> MMKIVVNNQSTLAAELMIVAQENLQKLVEQTKCPNSKALLDRRIFKAKSGEVLPLLHGDKIVILLGLGLRQDFIASEYDKIIAKAAEQLKKLAIKEISVDIDYAFENDNVKQFTLDTVRALISETYVFDQLKTEKENYSLEQIELVYSGDQDIEDSAKIGSAIACG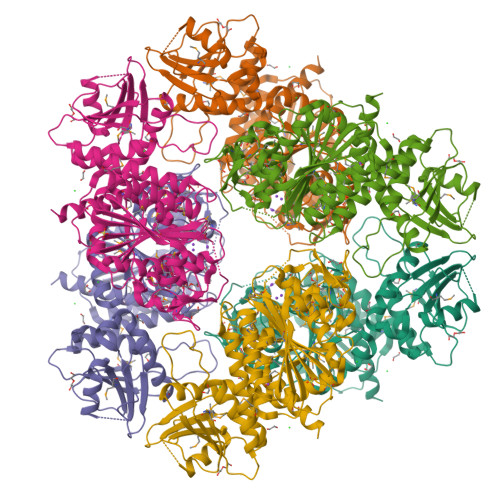QNYAKDLQNLPANICTTDYMLNEARELTSKYATFSLDYLDQDAMAELGMGCALAVGRGSYMSNYTVCMEYKGGNEGDAPIVLVGKGLVFDNGGICIKQAAGMDSMKMDMGGVAAVMGTMKAIAMLNLPVNVVGVMGLAENAVDARSYRPGDVLKSMKGITVEVSNTDAEGRLVLCDTLTYIGKYKPKAVIDLATLTGAMIISLGDAYSGMFANSDKLANSLEQAANASNDLIWRLPLHKPYLKKIESKVADMDNCGRDRSAGSIVAALFLSKFTEDYEWAHLDIAGSAMGDFASCKASGRPVPLLVHYLISQAKENLYFQ>[4x]GSHMRIAQVAPLWERVPP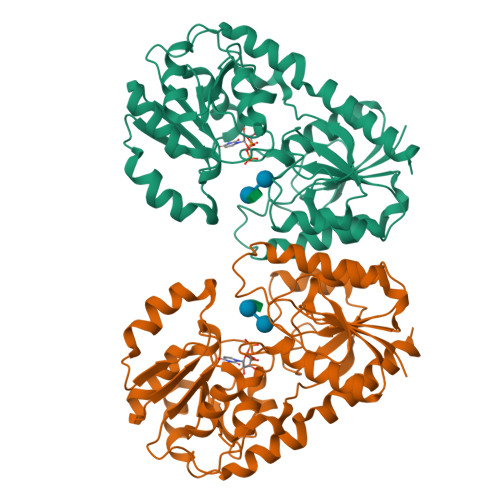PAYGGVELVVSLLTEELVKRGHEVTLFASGDSMTQAKLVSTYPHAIRLDPNVQEYAVYEALQLGEVFSRANEFDVIHSHVGYTALPYTSLVKTPVVHTLHGRFTADNERIFSQYRNQNYVSISHSQRQLRELNYIATVYNAIAVETHHFYPQPSDPPYLAFLGRLSPEKGPHHAIEIAKRVGIPLRMAGKVDRVDRDYFKELIEPHIDGEFIQFIGEADHPTKNALLGGAIAMLFPITWQEPFGLVMIESMAAGTPVVAIAKGAAPEVIEHGKTGFLCHSVEDCVAAVAQVPQLDRMACRDYVWQRFSVERMVSEYEAVYDTVLANTFVHNGHRRGTIELMAS[[(2R,5S)-5-(4-azanyl-5-fluoranyl-2-oxidanylidene-pyrimidin-1-yl)-1,3-oxathiolan-2-yl]methoxy-oxidanyl-phosphoryl] phosphono hydrogen phosphate | 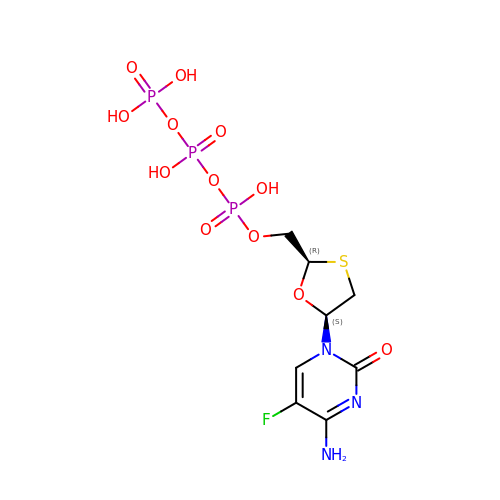C8 H13 F N3 O12 P3 S | WIEOLFZNMKSGEX-NTSWFWBYSA-N>MATMYKPSGNKRVTFKDVGGAEEAIEELKEVVEFLKDPSKFNRIGARMPKGILLVGPPGTGKTLLARAVAGEANVPFFHISGSDFVELFVGVGAARVRDLFAQAKAHAPCIVFIDEIDAVGRHRGAGLGGGHDEREQTLNQLLVEMDGFDSKEGIIVMAATNRPDILDPALLRPGRFDKKIVVDPPDMLGRKKILEIHTRNKPLAEDVNLEIIAKRTPGFVGADLENLVNEAALLAAREGRDKITMKDFEEAIDRVIAGPARKSLLISPAEKRIIAYHEAGHAVVSTVVPNGEPVHRISIIPRGYKALGYTLHLPEEDKYLVSRNELLDKLTALLGGRAA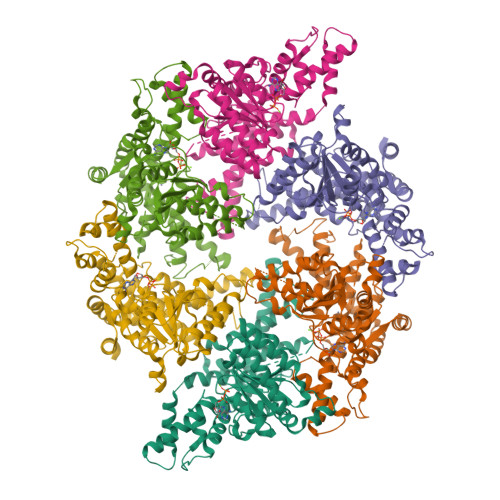EEVVFGDVTSGAANDIERATEIARNMVCQLGMSEELGPLAWGKEEQEVFLGKEITRLRNYSEEVASKIDEEVKKIVTNCYERAKEIIRKYRKQLDNIVEILLEKETIEGDELRRILSEEFEKVVEAAALEHHHHHH[6x]>[2x]MAQARKIPLDLPGTRILNGANWANNSATENLATNSGTLIIFDQSTPGQDA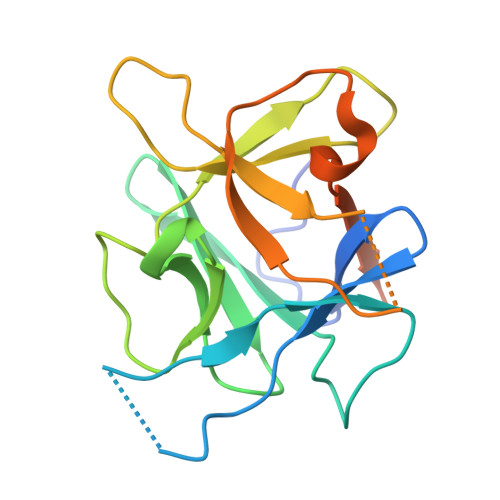DRWLIHNYLDGYKIFNMGSNNWASVSRGNTVLGVSEFDGQTCKWSIEYSGNGEEFWIRVPREGGGGAVWTIKPASSQGPTTVFLDLLKETDPNQRIKFAVDPNSSVDKLAAALEHHHHHH> 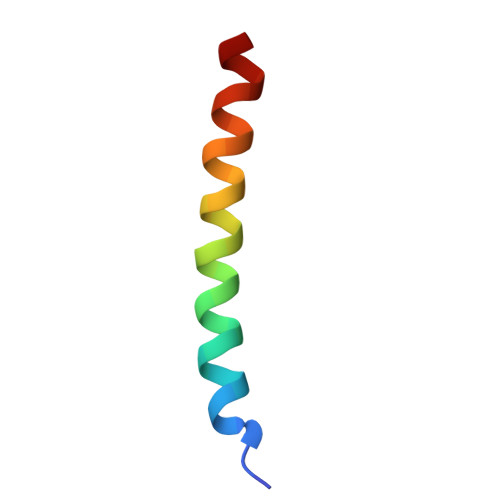MERSTRELCLNFTVVLITVILIWLLVRSYQY>MRSNLLAFSIVASLGLAQVAHAA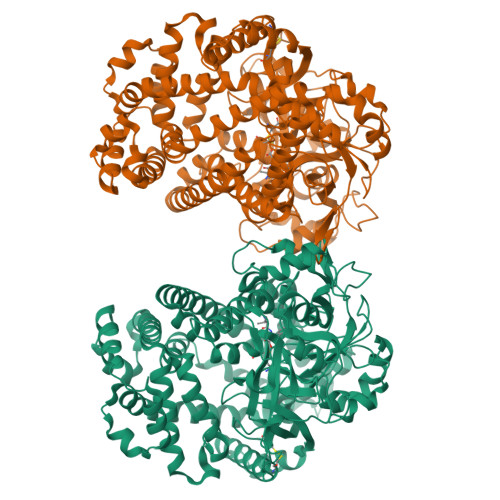EGMWVPQQLPEIAGPLQKAGLKLSPEQLANLTGDPMGAVVALGGCTASFVSPQGLVVTNHHCAYGAIQLNSTAQKNLIKDGFNAPTLKDELSAGPNARVFVLDQITDVTAQAKAAIAGAGNDPLARSRALDAFDKAQVAACEADAGFRCRLYSFSGGNTYRLFRNMEIKDVRLVYAPPGSVGKFGGDVDNWMWPRHTGDFSFYRAYVGKDGKPAAFAADNVPYQPKHFLKFADQPLGADDFVMVAGYPGRTNRYALAGEFNETASFTYPTIAKHYNAVLKMIADAGKADADVKVKYAATAASMNNVAKNYLGQLEGFKRIDAAGQKQAEEAAVLAWLKKQGAAGKPALAAHAQLLKHLDTSKSTRERDLFVGQFNNTSAVGAAITLYRLSIERSKPDAEREAGYQERDLTTIEGGLKQMDRRYVAKMDQQLQTYWLDQYVALPAAQRDNEVLNKWLAGSDAAAVKSLVNKLGGTELGSLDTRLKWFKADRAAFEASNDPAIQYAVAVMPALLKQEEQKKIREGESLTARPLYLQAVADYKKSQGEFVYPDANLSLRITFGNVMGYGKDGVKYTPFTTLEGVAAKETGEDPFDSPKALLDAVKAKRYGGLEDKRLGSVPVNFLSNLDITGGNSGSPVLDANGKLVGLAFDGNWESVSSNWVFDPVMTRMIAVDSRYMQWIMQEVAPAPQLLKELNLAK[2x]>GKLKKKGYLRIVTTQGSLNIELHADMAPRACDSFLRLCAVKYFDDTIFHRCIRNFMIQGGRAELRQPSKKKEVQQSPRSISGFPGGAPFEDEFDNRLVHQGIGVLSMANDGKHSNLSEFFITFKSCEHLNNKHTIFGRVVGGLDVL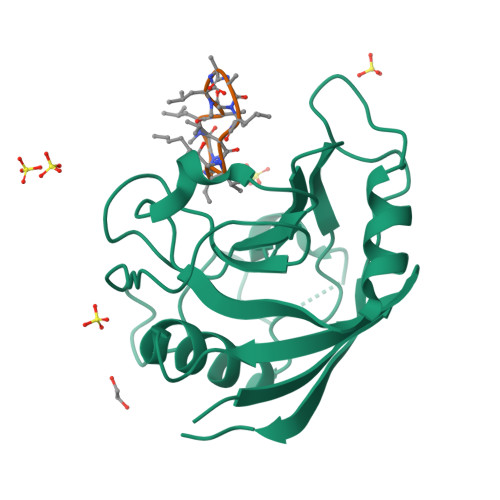RQWEKLETDKKDKPLKPPKVEEIIVFKNPFEDARKEMEDEKREEEEKEKKKLENA[4x];>ALLVTAGLVLA[4x]> NNLQNIIYNPVIPFVGTIPDQLDPGTLIVIRGHVPSDADRFQVDLQNGSSMKPRADVAFHFNP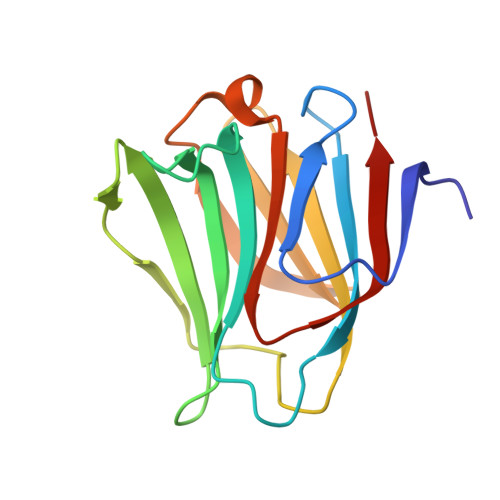RFKRAGCIVCNTLINEKWGREEITYDTPFKREKSFEIVIMVLKDKFQVAVNGKHTLLYGHRIGPEKIDTLGIYGKVNIHSIGFSFSSD> GGGAAGAUACAAG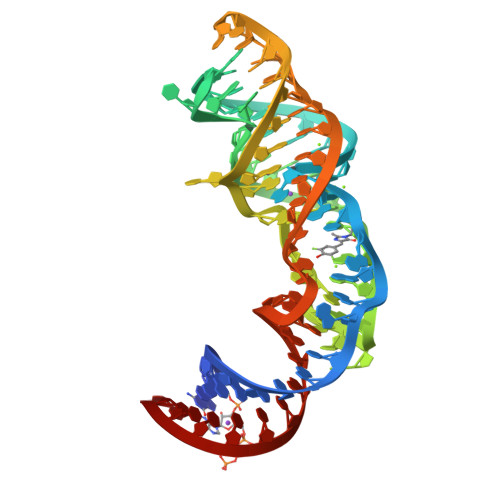GUGAGCCCAAUAAUAUGGUUUGGGUUAGGAUAGGAAGUAGAGCCUUAAACUCUCUAAGCGGUAUCUUCCC>MEIGFTFLDEIVHGVRWDAKYATWDNFTGKPVDGYEVNRIVGTYELAESLLKAKELAATQGYGLLLWDGYRPKRAVNCFMQWAAQPENNLTKESYYPNIDRTEMISKGYVASKSSHSRGSAIDLTLYRLDTGELVPMGSRFDFMDERSHHAANGISCNEAQNRRRLRSIMENSGFEAYSLEWWHYVL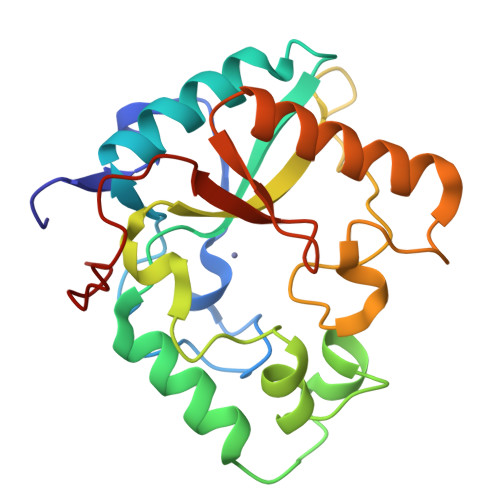RDEPYPNSYFDFPVK[6x]>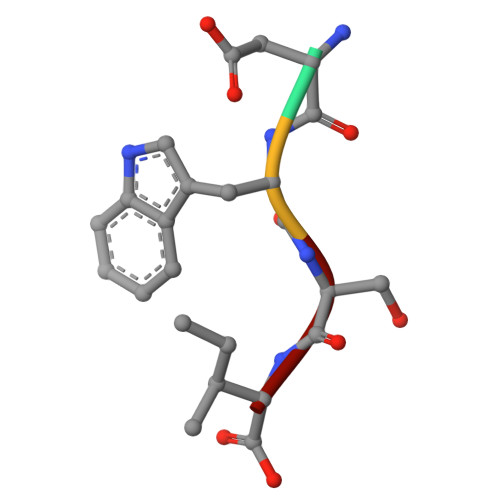 DWSI>[2x]MTRLFMLVCLGIVCQGTTGNILRGESLNKSLPILHEWKFFDYDFGSDERRQDAILSGEYDYKNNYPSDIDQWHDKIFVTMLRYNGVPSSLNVISKKVGDGGPLLQPYPDWSFAKYDDCSGIVSASKLAIDKCDRLWVLDSGLVNNTQPMCSPKLLTFDLTTSQLLKQV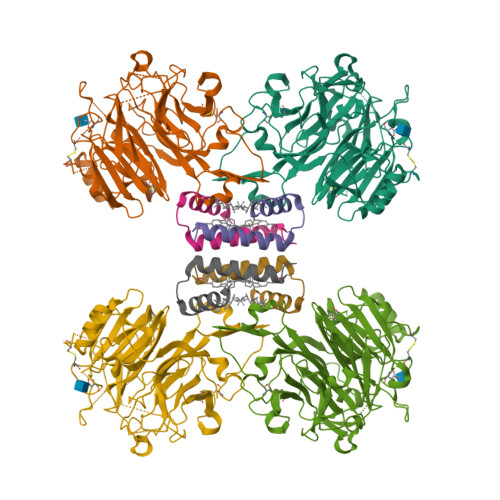EIPHDVAVNATTGKGRLSSLAVQSLDCNTNSDTMVYIADEKGEGLIVYHNSDDSFHRLTSNTFDYDPKFTKMTIDGESYTAQDGISGMALSPMTNNLYYSPVASTSLYYVNTEQFRTSDYQQNDIHYEGVQNILDTQSSAKVVSKSGVLFFGLVGDSALGCWNEHRTLERHNIRTVAQSDETLQMIASMKIKEALPHVPIFDRYINREYILVLSNKMQKMVNNDFNFDDVNFRIMNANVNELILNTRCENPDNDRTPFKISIHL;>MSKIVAVVVLAAFCVAMLVSDVSAKTSISVKGESNVDVVSQINSLVSSIVSGANVSAVLLAQTLVNILQILIDANVFA[2x]>AQDMVSPPPPIADEPLTVNTGIYLIECYSLDDKAETFKVNAFLSLSWKDRRLAFDPVRSGVRVKTYEPEAIWIPEIRFVNVENARDADVVDISVSPDGTVQYLERFSARVLSPLDFRRYPFDSQTLHIYLIVRSVDTRNIVLAVDLEKVGKNDDVFLTGWDIESFTAVVKPANFALEDRLESKLDYQLRISRQYFSYIPNIILPMLFILFISWTAFWSTSYEANVTLVVSTLIAHIAFNILVETNLPKTPYMTYTGAIIFMIYLFYFVAVIEVTVQHYLKVESQPARAASITRASRIAFPVVFLLANIILAFLFFGF[5x]

Pentameric ligand-gated ion channels are major mediators of fast synaptic transmission in the mammalian nervous system and serve a variety of biological roles across evolution. The extracellular domain (ECD) of each subunit contains β-strands β1–β10, with the characteristic Cys- or Pro-loop connecting β6–β7, and loops A–F enclosing a canonical ligand-binding site at the interface between principal and complementary subunits. The transmembrane domain (TMD) contains α-helices M1–M4, with M2 lining the channel pore, and an intracellular domain of varying length (2–80 residues) inserted between M3 and M4. GLIC has been thoroughly documented as a proton-gated ion channel, conducting currents in response to low extracellular pH with half-maximal activation around pH 5 (8).

Taking advantage of the flexible buffer conditions accessible to cryo-EM, we obtained additional reconstructions under partial and maximal (pH 5 and pH 3) activating conditions, producing maps to 3.4 and 3.6 Å, respectively. Surprisingly, backbone alignments of models at both pH 5 and pH 3 indicated close fits to the pH-7 model (root mean-squared deviation over non-loop Cα atoms, Root mean-squared deviation [RMSD] ≤ 0.6 Å) in both the ECD and TMD, including a closed conformation of the transmembrane pore. At pH 7 and pH 5, little definitive density was associated with this side chain (left, center); conversely at pH 3, it clearly extended towards the complementary loop F, forming a possible hydrogen bond with T158 (3.5 Å donor–acceptor). At the midpoint of the same β1–β2 loop, density surrounding basic residue K33 was similarly absent at pH 7 and pH 5, but clearly defined a side chain oriented down towards the TMD at pH 3. Conversely, at pH 5 and pH 3, K248 reoriented out towards the complementary subunit. Residue K248 has been implicated in GLIC ECD-TMD coupling, while E243 was shown to be an important proton sensor; indeed, rearrangement of K248 to an interfacial orientation is also evident in open X-ray structures, with an accompanying iris-like motion of the M2–M3 region—including both K248 and E243—outward from the channel pore. Interestingly, loop F adopted a different conformation in our structures at pH 5 compared to pH 7 or pH 3, suggesting this region samples a range of conformations; indeed, previous spin-labeling studies indicated this position, along with several neighbors on the β8 strand, to be highly dynamic. Thus, side chain arrangements in both the ECD and TMD were consistent with proton activation, while maintaining a closed pore.>MSTEASRSGKQEVDLTNCDREPIHIPGAIQPHGVLLVLSEPGLVLTHASENAPAVLGNSAEQLLGAPLGHFIEPSVREPLEADLRSARLKQLNPLKVVWRVDGVDRFFDGIAHRHQGRLILELEPSSHREAVPFLSFFHAVRDGLSRLRDARDLQELCEAVVQEVRGLTGFDRAIIYRFDAEWNGSVIAEARDARADPYLGLHFPASDIPRQARELYQLNWLRIIPTIDYQPARVRALPGHGEPLDLSFSVLRSVSPIHLEYLHNMGVQASMSISLMKDGKLWGLISCHQVSGTRYVPYEVRTACEFLGEVMSSLLAAKEGNEDYDQRIRAKSIHAALLERMAREVDFVSGLASQESGLLELVHAHGAAIHFHGRTTVLGQAPSDEALTGLIEWLGSRTGEGVFCTDRLAREYPEAQAFQEVAAGLMAFSMSRGRNNFVL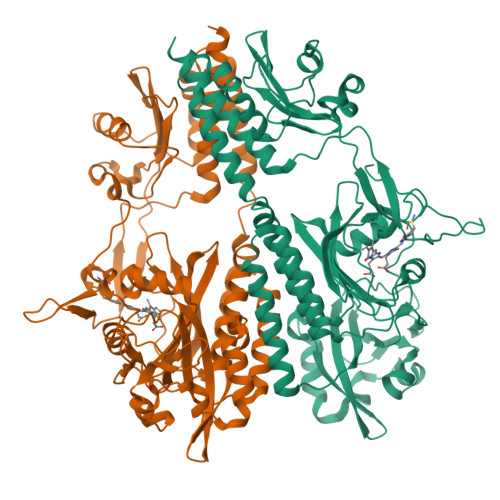WFRPEAVQTVNWSGNPTKAVEFDQGGPRLHPRKSFELWKETVRGRCLPWKAYEVEAASELRRSIIDVALQRSEEL[3x]>MEGGGKPNSSSNSRDDGNSVFPAKASATGAGPAAAEKRLGTPPGGGGAGAKEHGNSVCFKVDGGGGGGGGGGGGEEPAGGFEDAEGPRRQYGFMQRQFTSMLQPGVNKFSLRMFGSQKAVEKEQERVKTAGFWIIHPYSDFRFYWDLIMLIMMVGNLVIIPVGITFFTEQTTTPWIIFNVASDTVCLLDLIMNFRTGTVNEDSSEIILDPKVIKMNYLKSWFVVDFISSIPVDYIFLIVEKGMDSEVYKTARALRIVRFTKILCLLRLLRLSRLIRYIHQWEEIFHMTYDLASAVVRIFNLIGMMLLLAHWDGCLQFLVPLLQDFPPDCWVSLNEMVNDSWGKQYSYALFKAMSHMLCIGYGAQAPVSMSDLWITMLSMIVGATCYAMFVGHATALIQSLDSSRRQYQEKYKQVEQYMSFHKLPADMRQKIHDYYEHRYQGKIFDEENILNELNDPLREEIVNFNCRKLVATMPLFANADPNFVTAMLSKLRFEVFQPGDYIIREGAVGKKMYFIQHGVAGVITKSSKEMKLTDGSYFGEICLLTKGRRTASVRADTYCRLYSLSVDNFNEVLEEYPMMRRAFETVAIDRLDRIGKKNSILLQKFQKDLNTGVFNNQENEILKQIVKHDREMVQAIAPINYPQMTTLNSTSSTTTPTSRMRTQSPPVYTATSLSHSNLHSPSPSTQTPQPSAILSPCSYTTAVCSPPVQSPLAARTFHYASPTASQLSLMQQQPQQQVQQSQPPQTQPQQPSPQPQTPGSSTPKNEVHKSTQALHNTNLTREVRPLSASQPSLPHEVSTLISRPHPTVGESLASIPQPVTAVPGTGLQAGGRSTVPQRVTLFRQMSSGAIPPNRGVPPAPPPPAAALPRESSSVLNTDPDAEKPRFASNL[4x]

Hyperpolarization and cyclic nucleotide (HCN) activated ion channels are critical for the automaticity of action potentials in pacemaking and rhythmic electrical circuits in the human body. Unlike most voltage-gated ion channels, the HCN and related plant ion channels activate upon membrane hyperpolarization. HCN channels are also regulated by cyclic nucleotides, which act via the CNBD and fine-tune the frequency of their pacemaking activity. Here, we present cryo-electron microscopy structures of human HCN1 corresponding to Closed, Open, and a putative Intermediate state.

To investigate the role of these cysteines further, we solved the structure of the HCN1-F186C-S264C-C309A mutant in the presence of Hg2+ and an identical LMNG:lipid:CHS ratio to a global resolution of 3.6 Å. Based on the position of the S4 and S5 helices, we classify this as the Intermediate-state structure. Mutation of C309 to alanine results in an intermediate state with closed pore supporting the notion that—at least structurally—this bond is stabilizing the Open-state structure. A comparison of the voltage-sensing domains in the three HCN channel structures reveals that in the Intermediate state, the R4 charge of the S4 helix moves past the Cα position of the charge transfer center F186 by a quarter helical turn. While the resolution at the intracellular end of the S4 helix in the Intermediate state precludes definitive assignment of secondary structure, the weaker density at the C-terminal end suggests that it may be on the pathway to unraveling. In both the Closed and Intermediate structures, the diameters of the pore gate are below 1.0 Å, too small to allow passage of ions. While the Intermediate structure shows a marginal increase in the diameter of the cavity and narrowing of the gate and selectivity filter, there is no noticeable rotation of the S6 transmembrane helices. Strikingly, in the Intermediate and Open-state structures, the intracellular helix–turn–helix region between I284 and V296 becomes unwound, suggesting that voltage-sensor activation destabilizes this gating interface. Interestingly, we observe far fewer lipid densities in this Intermediate structure, with only 1–2 prominent densities at the S5–S6 interface than in the Closed state. Finally, it is worth noting that in both Open and Intermediate structures, we observe only weak densities corresponding to the N-terminal HCN domain, suggesting that interactions with this domain and the S4 helix or CNBD are weakened upon activation.Members of glycosyltransferase family 75 (GT75) not only reversibly catalyze the autoglycosylation of a conserved arginine residue with specific NDP-sugars but also exhibit NDP-pyranose mutase activity that reversibly converts specific NDP-pyranose to NDP-furanose. MtdL from deep sea–derived Marinactinospora thermotolerans SCSIO 00652 has been discovered in the antibiotic A201A biosynthetic pathway, generating GDP-L-galactofuranose (L-Galf) from GDP-L-galactopyranose (L-Galp). The MtdL subunit is divided into three regions: the N-terminal region (residues 1–111), the core region (residues 112–291), and the C-terminal region (residues 292–376). The characteristic DXD motif (Asp109-Asp110-Asp111), together with conserved His287, coordinates a Mn2+ ion, which stabilizes the diphosphate of the nucleotide.

To obtain the Mn2+·GDP-L-Fucp complex structure, we initially soaked the crystal of MtdL containing 0.5 mM MnCl2 with 5 mM GDP-L-Fucp. However, no electron density of the L-Fucp moiety was observed, possibly due to enzymatic catalysis toward GDP-L-Fucp. Then, the S228A mutant with decreased enzymatic activity was used for crystallization. The complex structure of MtdL-S228A·Mn2+·GDP-L-Fucp at 2.2-Å resolution was obtained by soaking the crystal of MtdL-S228A containing 0.5 mM MnCl2 with 5 mM GDP-L-Fucp and 0.5 mM MnCl2. The electron density for Mn2+ and the L-Fucp moiety could be seen in this structure. Asp260 hydrogen bonds to the L-Fucp C2-OH, C3-OH, and C4-OH, simultaneously. Besides, the L-Fucp C2-OH hydrogen bonds to the side chains of Arg159 and Gln229. Arg159 is located closer than Arg257 to the anomeric carbon with a distance of 3.9 and 4.3 Å, respectively, in the GDP-L-Fucp complex structure. We noted that L-Fucp C4-OH is positioned at a hydrogen bond distance (3.1 Å) with the carboxyl group of Asp260 in the MtdL·Mn2+·GDP-L-Fucp complex structure, whereas the D-Glcp C4-OH is positioned with a distance of 3.8 Å to the carboxyl group of Asp260 in the MtdL·Mn2+·GDP-D-Glcp complex structure. The shorter distance of L-Fucp C4-OH compared with that of D-Glcp C4-OH to the putative catalytic base might dictate the mutase activity of MtdL toward GDP-L-Fucp instead of GDP-D-Glcp.

>[2x]GSSHHHHHHSSGENLYFQHMSGRDISTAVVVTTISDGGFLDRLAPALRDAGARLIVIPDRNTGPALFAACERHRRLGLDVVCPSVAEQQDLLERLAVPDLIPYHSDNRRNVGYLMAWMEGFDVIVSMDDDNLPTTDDFVERHQVVCQGPRTQPVTASSDGWFNNCALLEVEPTEVFPRGFPFHARPAHAQARTSVCERPADVRINAGLWLGDPDVDAITRLAVRPNALAHSGGSVVLAEGTWCPVNAQNTAVHRDALPAYYFLRMGQPVDGVPMERFGDIFSGYFVQVCAQHLGHAVRFGDPVVEHPRNEHDLLDDLHKEVPAVRLLDDILDHLRDHPLEGGDYLETYESLSYALQEIAERVNGRAWSPDARAFLHRSAHLMRSWTGALRTVAGT>[4x]MSLRAVRLHAKWDPRPEFKLGPKDIEGKLTWLGSKVWRYPEVRVEEVPEPRIEKPTEIIIKVKACGICGSDVHMAQTDEEGYILYPGLTGFPVTLGHEFSGVVVEAGPEAINRRTNKRFEIGEPVCAEEMLWCGHCRPCAEGFPNHCENLNELGFNVDGAFAEYVKVDAKYAWSLRELEGVYEGDRLFLAGSLVEPTSVAYNAVIVRGGGIRPGDNVVILGGGPIGLAAVAILKHAGASK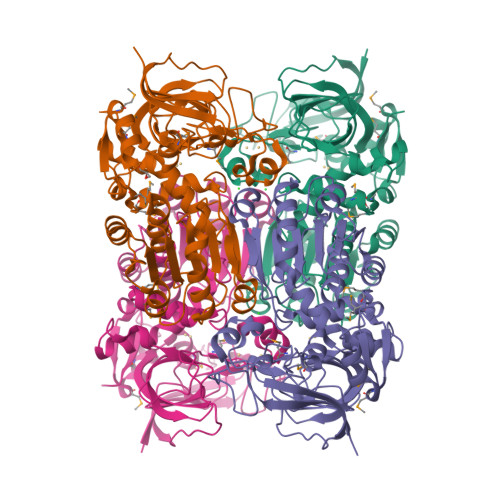VILSEPSEVRRNLAKELGADHVIDPTKENFVEAVLDYTNGLGAKLFLEATGVPQLVWPQIEEVIWRARGINATVAIVARADAKIPLTGEVFQVRRAQIVGSQGHSGHGTFPRVISLMASGMDMTKIISKTVSMEEIPEYIKRLQTDKSLVKVTMLNEGHHHHHH>MVANPEHYIKHPLQNRWALWFFKNDKSKTWQANLRLISKFDTVEDFWALYNHIQLSSNLMPGCDYSLFKDGIEPMWEDEKNKRGGRWLITLNKQQRRSDLDRFWLETLLCLIGESFDDYSDDVCGAVVNVRAKGDKIAIWTTECENRDAVTHIGRVYKERLGLPPKIVIGYQSHADTATKSGSTTKNRFVV[4x]

In addition, the cap fulfills numerous other biological functions that are mediated by specific cap-binding proteins and include maturation, transport, and eIF4E-mediated translation initiation. Upon binding the cap, the eIF4E protein changed its conformation from open to closed, bringing the Trp102 and Trp56 closer to the cap, and together with the structural water molecules, stapling the ligand with the protein structure. Finally, to gain more insight into the consequences at the molecular level of N7-benzylation of the mRNA cap, we determined the crystal structures of three compounds with eIF4E. Overall, the comparison of these three crystal structures indicated that different benzyl substituents can be accommodated in the cap binding pocket due to (i) the conformational flexibility of Trp102, which was also previously observed for m7GMP analogs, and (ii) the presence of structural water molecules in the N7-methyl-binding cavity, which could be replaced upon introduction of larger hydrophobic substituents.

Crystal structures were refined using diffraction data to the resolution of 2.2 Å for 1a, 2.67 Å for 1c, and 2.66 Å for 1h. Finally, the electron density for the complex with the 4-chlorobenzyl dinucleotide (1h) indicated that the Trp102 could adapt two conformations—the one similar to that in the complex with m7GpppG, with the nitrogen atom directed towards the cap binding site, and the second flipped by 180° with the nitrogen atom directed towards the solution (similar to that observed for 1c). In the case of the benzyl modified cap 1a, for which the benzyl ring was directed upwards, most of the structural water molecules were conserved in the cavity, while for 3-MeBn7GpppG and 4-Cl-Bn7GpppG the benzyl rings were directed downwards into the cavity, and the structural water molecules were replaced by 3-methylbenzyl rings or 4-chlorobenzyl substituents. In the eIF4E complex with 1h one structural water molecule was conserved, which together with the hydroxyl group of Ser92 appeared to form polar contacts with the chlorine atom. For the eIF4E complex with 4-Cl-Bn7GpppG (1h), in which 4-chlorobenzyl appeared to be stabilized via polar contacts in the cavity, the phosphate chain could adopt two conformations, wherein one imitated the phosphate chain of m7GpppG, while in the Bn7GpppG (1a) and 3-MeBn7GpppG (1c) complexes, γ and β phosphates were shifted out of the pocket by 2–3 Å (distances measured between corresponding phosphorus atoms). The guanosine of 4-Cl-Bn7GpppG was not visible in the crystal structure, while the guanosines of Bn7GpppG and 3-MeBn7GpppG were stabilized by interactions with amino acids from the loop comprised of residues 50–59. Single halogen substitutions at the para position (1g, 1h, 1i) did not disrupt and even slightly stabilized the complex, whereas double substitutions (1j, 1k) destabilized the complex, probably due to steric hindrance.URIDINE-5'-DIPHOSPHATE-N-ACETYLMURAMOYL-L-ALANINE | C23 H36 N4 O20 P2 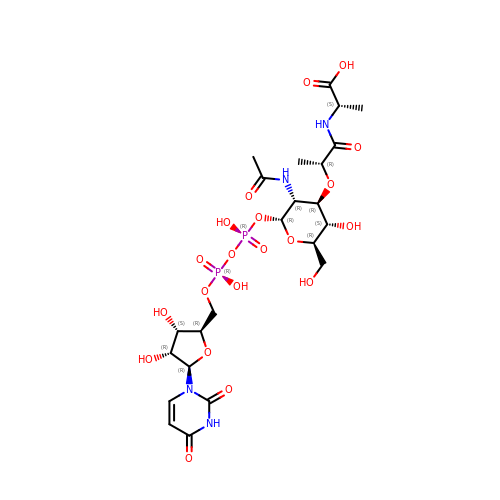| NTMMCWJNQNKACG-KBKUWGQMSA-N1,3-dimethyl-6-(2-methylpropoxy)pyrimidine-2,4(1H,3H)-dione 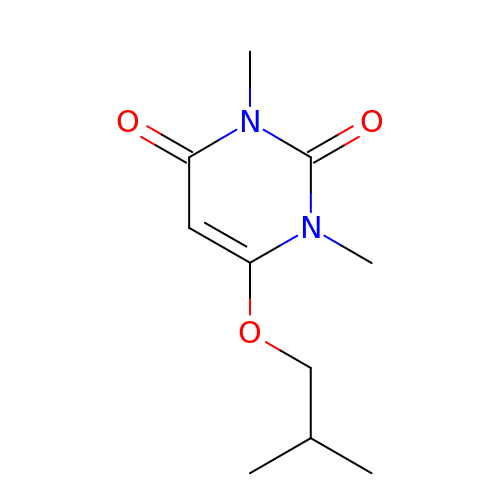| C10 H16 N2 O3 | NBDGERYKSQRETJ-UHFFFAOYSA-N> MAFLDNPTIILAHIRQSHVTSDDTGMCEMVLIDHDVDLEKIHPPSMP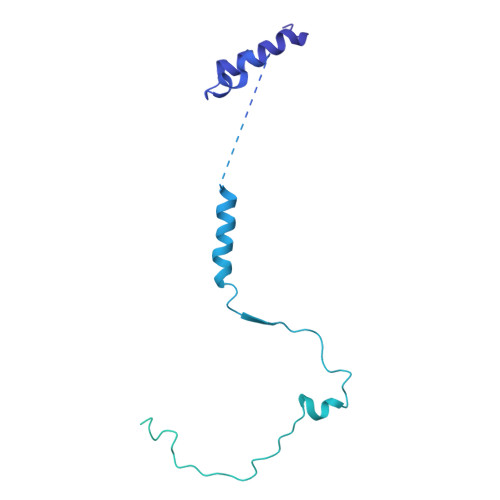GDSGSEIQGSNGETQGYVYAQSVDITSSWDFGIRRRSNTAQRLERLRKERQNQIKCKNIQWKERNSKQSAQELKSLFEKKSLKEKPPISGKQSILSVRLEQCPLQLNNPFNEYSKFDGKGHVGTTATKKIDVYLPLHSSQDRLLPMTVVTMASARVQDLIGLICWQYTSEGREPKLNDNVSAYCLHIAEDDGEVDTDFPPLDSNEPIHKFGFSTLALVEKYSSPGLTSKESLFVRINAAHGFSLIQVDNTKVTMKEILLKAVKRRKGSQKVSGPQYRLEKQSEPNVAVDLDSTLESQSAWEFCLVRENSSRADGVFEEDSQIDIATVQDMLSSHHYKSFKVSMIHRLRFTTDVQLGISGDKVEIDPVTNQKASTKFWIKQKPISIDSDLLCACDLAEEKSPSHAIFKLTYLSNHDYKHLYFESDAATVNEIVLKVNYILESRASTARADYFAQKQRKLNRRTSFSFQKEKKSGQQ>[8x]SSE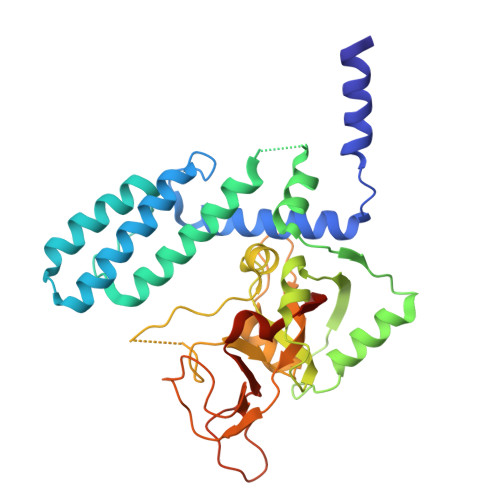QLQALLLEEVMNSSTLSQEVSDLVEMIWAEALGHLEHMLLKPVNRISLNDVSKAEGILLLVKAALKNGETAEQLQKMMTEFYRLIPHKGTMPKEVNLGLLAKKADLCQLIRDMVNVCETNLSKPNPPSLAKYRALRCKIEHVEQNTEEFLRVRKEVLQNHHSKSPVDVLQIFRVGRVNETTEFLSKLGNVRPLLHGSPVQNIVGILCRGLLLPKVVEDRGVQRTDVGNLGSGIYFSDSLSTSIKYSHPGETDGTRLLLICDVALGKCMDLHEKDFSLTEAPPGYDSVHGVSQTASVTTDFEDDEFVVYKTNQVKMKYIIKFSMPGDQIKD>[2x]VVGGF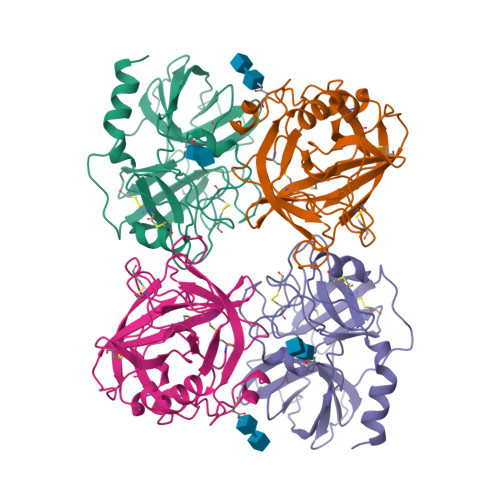NCEKNSQPWQVAVYYQKEHICGGVLLDRNWVLTAAHCYVDQYEVWLGKNKLFQEEPSAQHRLVSKSFPHPGFNMSLLMLQTIPPGADFSDDLMLLRLSKPADITDVVKPIALPTKEPKPGSKCLASGWGSITPTRWQKPDDLQCVFITLLPNENCAKVYLQKVTDVMLCAGEMGGGKDTCRDDSGGPLICDGILQGTTSYGPVPCGKPGVPAIYTNLIKFNSWIKDTMMKNA>[4x]MEMKKSGLGTTAIHAGTLKNLYGTLAMPIYQTSTFIFDSAEQGGRRFALEEAGYIYTRLGNPTTTVLENKIAALEEGEAGIA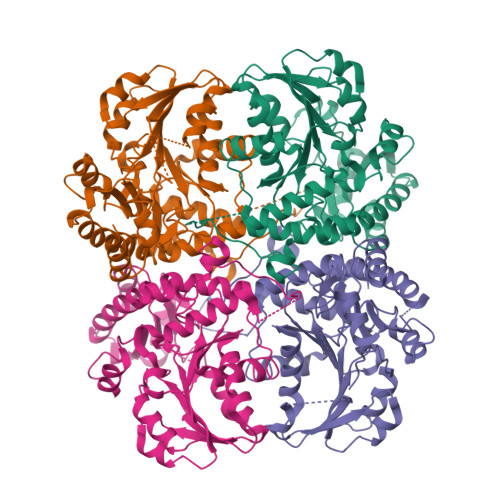MSSGMGAISSTLWTVLKAGDHVVTDKTLYGCTFALMNHGLTRFGVEVTFVDTSNLEEVKNAMKKNTRVVYLETPANPNLKIVDLEALSKIAHTNPNTLVIVDNTFATPYMQKPLKLGVDIVVHSATKYLNGHGDVIAGLVVTRQELADQIRFVGLKDMTGAVLGPQEAYYIIRGLKTFEIRMERHCKNARTIVDFLNKHPKVEKVYYPGLETHPGYEIAKKQMKDFGAMISFELKGGFEAGKTLLNNLKLCSLAVSLGDTETLIQHPASMTHSPYTKEEREVAGITDGLVRLSVGLENVEDIIADLEQGLEKI> LFNEIIPLGRLIHMVNQKKDRLLNEYLSPLDITAAQFKVLCSIRCAAC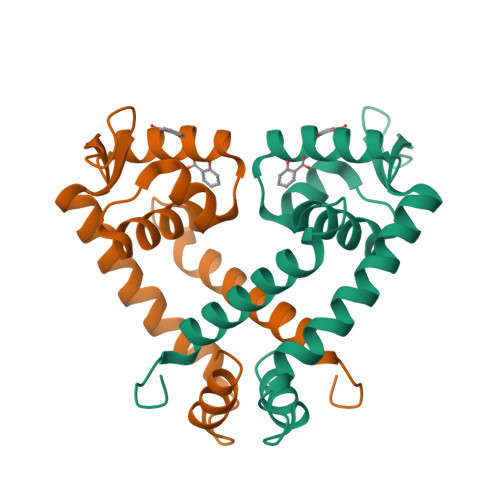ITPVELKKVLSVDLGALTRMLDRLVCKGWVERLPNPNDKRGVLVKLTTGGAAICEQCHQLVGQDLHQELTKNLTADEVATLEYLLKKVLP> MNMLVINGTPRKHGRTRIAASYIAALYHTDLIDLSEFVLPVFNGEAEQSELLKVQELKQRVTKADAIVLLSPEYHSGMSGA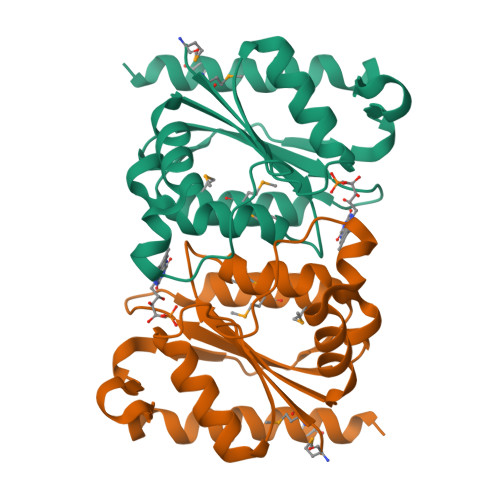LKNALDFLSSEQFKYKPVALLAVAGGGKGGINALNNMRTVMRGVYANVIPKQLVLDPVHIDVENATVAENIKESIKELVEELSMFAKAGNPGV At the parasite–host interface, F. hepatica calcium-binding proteins (FhCaBPs) have a unique EF-hand/DLC-like domain fusion found only in trematodes. A unique family of proteins called calcium-binding protein (CaBPs) or tegumental allergen-like (TALs) proteins are abundant in trematodes. These proteins have a dynein light chain (DLC)-like domain at the C-terminal and a calmodulin-like domain with an EF-hand motif at the N-terminal. Among the F. hepatica paralogs, FhCaBP4 is notable because unlike other proteins in this group, it exhibits calcium-dependent dimerization and increases hydrophobic surface exposure upon calcium ion binding.

We successfully determined the crystal structure of the apo form at 1.93 Å resolution. The asymmetric unit contained two FhCaBP4 molecules forming a homodimer with a two-fold axis. Each FhCaBP4 monomer consists of an N-terminal calmodulin-like domain (residues 4–90) connected via a 10-residue flexible hinge to a C-terminal dynein light chain (DLC)-like domain (residues 101–190). The α1 to α4 helices form classical EF-hand motifs, where two helix–loop–helix structures are connected by two short antiparallel β-sheets (β1 and β2) that flank the Ca2+-binding loops. The DLC-like domain adopts a compact β-sandwich fold composed of antiparallel β-strands (β3, β5, β6, β4) capped by an α6/α7 helical hairpin.Sequence conservation analysis revealed that the EF-hand motifs are genetically conserved, whereas the flexible linker region is not, suggesting that this region may confer species-specific flexibility and functional diversity. Five residues (W163 to S167) of each protomer in the extended loop interact with five residues (Q’154 to V’157) of the neighboring protomer in the β4-strand through a pair of hydrogen bonds. Superposition with the FhCaBP2 DLC-like domain model (5XF0) yielded an RMSD of 1.45 Å over 88 Cα atoms in PyMOL and 1.0 Å with a Z-score of 16.1 for 87 Cα atoms in DALI, highlighting strong conservation within the FhCaBP family. However, a key deviation was found in the flexible loop between β4 and β5 (residues Phe166 to Phe171), which displayed significant conformational variability despite the conserved sequence. The elevated number of interactions in FhCaBP4, particularly those involving Glu12 and Glu78 located in helices α1 and α5, respectively, indicates that the calmodulin-like domain contributes to stabilizing the flexible loop within the DLC-like domain. The calmodulin-like domain exhibited an RMSD of 3.5 Å (79 Cα atoms, DALI Z-score 7.6), whereas the DLC-like domain remained structurally stable (RMSD 0.5 Å, 90 Cα atoms, DALI Z-score 20.0).

>MGEVALEGSNLEKMIQLFLQLDRNRDDIVDENELRQACAEHKLPEEEVSRWLDMFDADENGKITLEEFCRALGLRTAEMRVEKMEREEVRAGRGRPMPEDVEVIASTMSQEKKVEVTEKFKEFLAKTGGKPEDMNLVVKQLKDYLDERHGRVWQTLVLTGSYWMKFSHEPFMSLQFKVGPNIVLVWRTPSN[2x]>[2x]GHMNANLPPSAISELHGPRLLLRAWRDSDREAFAEMCADPQVMEFFPSVLDRAQSDALVDRVQAHFAERGYGPWALELPGEAAFIGFTGLFDVTMDVHFAPTVAIGWRLAPAYWGRGLAREAAETALDFAFERLRLPEVVAFTTPPNRRSWGLMERLGMRRDPAEDFDHPLLAADHPMRRHILYRVDAARWAER

Enzymes in the Gcn5-related N-acetyltransferase (GNAT) superfamily are widespread and critically involved in multiple cellular processes ranging from antibiotic resistance to histone modification. Previously, we determined the structure of the PA3944 GNAT enzyme from Pseudomonas aeruginosa and found that it could acetylate polymyxin antibiotics, specifically the 3-Dab residue on polymyxin B and on colistin. The canonical chemical mechanism attributed to GNATs is a general acid/base mechanism; however, mounting evidence has cast doubt on the applicability of this mechanism to all GNATs. This study shows that the Pseudomonas aeruginosa PA3944 enzyme uses a nucleophilic serine residue and a hybrid ping-pong mechanism for catalysis instead of a general acid/base mechanism. Instead, PA3944 has a serine (S148) in a comparable location as the typical critical tyrosine residue found in GNATs.

The only residue that could potentially act in this capacity was E102, so we mutated it to alanine and screened the enzyme for activity toward both polymyxin B and NANMO. Specifically, the catalytic efficiency decreased by one order of magnitude compared to WT when polymyxin B was the substrate, but increased by one order of magnitude compared to WT when NANMO was the substrate. Based on these results, it appears that E102 more likely plays a role in substrate specificity rather than in the catalytic mechanism. Since we observed a significant improvement in catalytic efficiency of the PA3944 E102A enzyme toward NANMO, we crystallized the protein to determine whether we would observe structural changes that might help explain the kinetic observations. There were minor perturbations in the positions of the flexible β3-β4 and β6-β7 loops between the mutant and WT protein backbones. The removal of the negative charge from the E102 side chain provided space for the orientation of the phenyl ring of F89 to flip inward compared to the WT structure 2. Additionally, the removal of the negative charge of E102 increased the overall hydrophobicity of the acceptor substrate binding site. The change in hydrophobicity combined with the conformational change of the F89 residue helps explain the improvement in apparent affinity of the E102A protein for NANMO compared to polymyxin B. When we examined the same docking studies but in the PA3944 E102A structure, we found the protonated NANMO in presence of AcCoA formed an H-bond with the backbone oxygen of F140 but the free base NANMO formed an H-bond with the backbone oxygen of F43. When we docked NANMO into the E102A structure, we found two additional residues that were located in close proximity to the molecule that were not observed in the WT docking: W105 and M152.>[2x]MCGGLHRDGTPAGPSAGCPRLTAAALSAGQDALGPSSETQELECALDFLRGSDDPALRRSSLGSRICLHLAERNSDPAERARFAREGVERAEAALAQGGEDDGAVHYYLAANLGLAVRDDMTAALANLHRLEHESEAAVKLSPDFDDGGPLRLLGMLYLKAPAWPAGMGDGDKALDLLGQAVERHPGHPLNHLFYAEALWEVNGESESRRVEEEMAAGWRLLESGSWGYNKQIWKREFADLRQEIGAPARLEHHHHHH

The aerobic methanotroph Methylococcus capsulatus was the first bacterium shown to synthesize sterols, producing a mixture of C-4 methylated sterols that are distinct from those observed in eukaryotes. C-4 methylated sterols are synthesized in the cytosol and localized to the outer membrane, suggesting that a bacterial sterol transport machinery exists. In this study, we present three putative bacterial sterol transport proteins in M. capsulatus that exhibit remarkable specificity for C-4 methylated sterols. We first used bioinformatics to identify a cytoplasmic membrane protein (BstA), periplasmic protein (BstB), and outer membrane associated protein (BstC).

Finally, BstC is predicted to be a T-component member of the tripartite ATP-independent periplasmic component superfamily, which comprises periplasmic lipoproteins implicated in the cytoplasmic import of small molecules. The structure of BstC was also determined by experimental phasing to a resolution of 1.9 Å. Two monomers (RMSD of 0.656 Å for all Cαs) in the asymmetric unit form a dimer with 180 rotational symmetry. Each monomer adopts an all-α-helical structure with 12 α-helices in total, designated with H1 to H12; 9 antiparallel arranged helices (H4-H12) form an irregular ring with a pore running through the center. Three cavities are found in the center of the structure. TN1 is closer to the N-terminal face of the structure, while CA1 and CA2 are proximal to the C-terminal face and form two open hydrophobic pockets; TN1 exhibits a mixture of hydrophobic and hydrophilic amino acids. All the sterols were found embedded in the hydrophobic cavity (CA1) lined by Gly128, Val131, Arg132, Met135, Ala138, Leu139, Leu142, Leu145, Leu167, Met170, Leu171, Lys174, Ala175, Pro176, and Phe208, with the hydroxyl group pointing inwards and the aliphatic tail pointed out. The simulations reveal that the substrate moves approximately 8–9 Å further into the binding site and the polar head makes a hydrogen bonding contact with the side chain of Glu86. Mutagenesis to convert Glu86 to Gly and Trp to remove or reduce the potential interactions with the polar head of the sterols leads to ~4.5 and 100-fold decrease in the equilibrium affinity for 4-monomethyl sterol. Size-exclusion chromatography coupled with multiangle light scattering (SEC-MALS) analysis shows that indeed the purified BstC exists both as a monomer and a dimer in solution with a ratio ~3:1.> GPVEDAITAAIGRVADTVGTG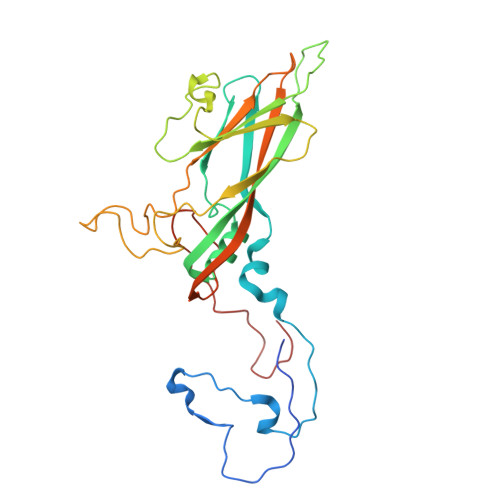PTNSEAIPALTAAETGHTSQVVPGDTMQTRHVKNYHSRSESTIENFLCRSACVYFTEYENSGAKRYAEWVLTPRQAAQLRRKLEFFTYVRFDLELTFVITSTQQPSTTQNQDAQILTHQIMYVPPGGPVPDKVDSYVWQTSTNPSVFWTEGNAPPRMSIPFLSIGNAYSNFYDGWSEFSRNGVYGINTLNNMGTLYARHVNAGSTGPIKSTIRIYFKPKHVKAWIPRPPRLCQYEKAKNVNFQPSGVTTTRQSITTMTNT> ENIIRIKDDNKAVSLGTSKINYIDPRIICSWAKAQDVPINKI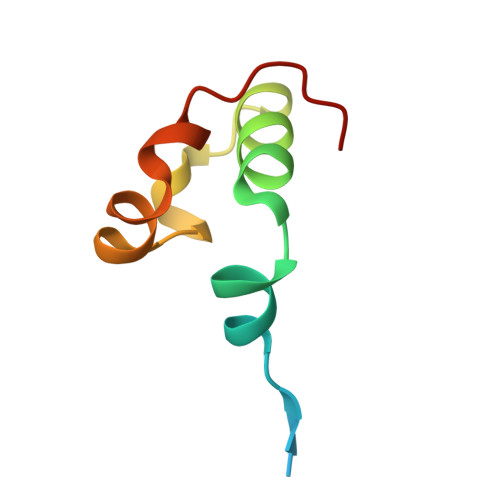FSATIQKKFPWAMNAENFDF>[2x]ADTKAKLTLDGDTAVELDVLKGTLGQDVIDIRT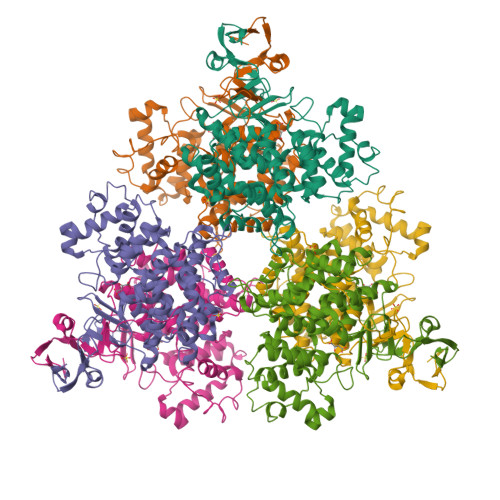LGSKGVFTFDPGFTSTTSCESKITFIDGDEGILLHRGFPIDQLATDSNYLEVCYILLNGEKPTQEQYDEFKTTVTRHTMIHEQITRLFHAFRRDSHPMAVMCGITGALAAFYHDSLDVNNPRHREIAAFRLLSKMPTMAAMCYKYSIGQPFVYPRNDLSYAGNFLNMMFSTPCEPYEVNPILERAMDRILILHADHEQNASTSTVRTAGSSGANPFACIAAGIASLWGPAHGGANEAALKMLEEIGKKENIPEFVRRAKDKNDSFRLMGFGHRVYKNYDPRATVMRETCHEVLKELGTKDDLLEVAMELENIALNDPYFIEKKLYPNVDFYSGIILKAMGIPSSMFTVIFAMARTVGWIAHWSEMHSDGMKIARPRQLYTGYEKRDFKSDIKR The major class of these adhesive pili (or fimbriae) is assembled via the classical, alternative and archaic chaperone-usher (CU) pathways. The biogenesis of CU fibres requires a periplasmic chaperone and outer membrane assembly platform termed the usher. Here, we report atomic-resolution insight into the structure and biogenesis of Acinetobacter baumannii Csu and Escherichia coli ECP pili assembled via the archaic and alternative pathways, respectively, whilst also highlighting some important deviations from the classical assembly mechanism. The non-classical chaperones, unlike their classical counterparts, maintain subunits in a substantially unfolded state by utilising a register-shifted DSC and a distinct subunit C-terminal carboxylate anchor.

ECP is composed of the EcpA and EcpD subunits, which are assembled using two periplasmic chaperones, EcpB and EcpE, and the EcpC usher. We next crystallized free EcpB and determined its structure using I-SIRAS phasing to 2.4 Å resolution. EcpB consists of the two characteristic Ig-like domains as seen in all other chaperones and has an overall boomerang-like shape. As expected, the superposition revealed that EcpB is structurally more related to CsuC (Z-score = 14.2) than classical chaperones (e.g. Caf1M, Z-score = 12.0). No topological differences were found in D1 between EcpB and CsuC, but both possess an additional strand D1 that is absent in the classical chaperones. Whereas the β-sheet packing in D2 in subunit-bound CsuC is almost orthogonal, in EcpB, the two β-sheets pack nearly parallel to each other, at an angle of just 15–30°. Domain 2 of EcpB does not possess helix 1, common in classical chaperones, or helices 1 and 2, characteristic for archaic chaperones. Instead, it has a short helix located in a long loop between β-strands C2 and D2. The C2-D2 loop is flanked with a pair of conserved cysteines (170 and 179), which form a disulphide bond that is not seen in classical chaperones. In contrast, the domain orientation in subunit-free conformations can be varied significantly, as seen in the structure of EcpB, which implies that a substantial rearrangement in the relative domain orientation occurs during the formation of the chaperone-subunit complex.

> MAHHHHHHVDDDDKMLDVGDISSFMNSDSSTLSKTIQNSTDSGRLINIRLERLSSPLDDGQVIAMDKPDELLLTPASLLLPAQASEVIRFFYKGPADEKERYYRIVWFDQALSDAQRDNANRSAVATASARIGTILVVAPRQANYHFQYANGSLTNTGNATLRILAYGPCLKAANGKECKENYYLMPGKSRRFTRVDTADNKGRVALWQGDKFIPVK> MDEKTKKAEEMALSLARAVAGGDEQAAIKYATWLAEQRVPLRVQVKPEVSPTQDIRLCVSVEDAYMHTVTIWLTVRPDMTVASLKDMVFLDYGFPPSLQQWVVGQRLARDQETLHSHGIRRNGDGAYLYLLSARNTSLNP;> GRQDKMRKEGLQLVSMIQEGETAGASPEEVFSALQYSGTEVPLQWLRSELSYVLEMVAELAGQQDPELGAFSCQEARKAWLDRHGNLDEAVEECVRARRRKVHELQSLGFGPKEGSLQALFQHGGDVARALTELQRQRLEPFHQRLWDRDPEPTPCWD;> GPLGSPEFSSGNFKKEELATRLSQAIAGGDEKAAAQVAAVLAQHHVALNVQLMEAWFPPGPIRLQVTVEDATSVLSSSSSAHVSLKIHPHCSIAALQDQVFSEFGFPPAVQRWVIGRCLCMPERSLASYGVSQDGDPAFLYLLSAPREVSGQSLQNSKMDRKLGLFPQSLGLPHDLQPSSSSLPSPS

The linear ubiquitin chain assembly complex (LUBAC) participates in inflammatory and oncogenic signaling by conjugating linear ubiquitin chains to target proteins. LUBAC consists of the catalytic HOIP subunit and two accessory subunits, HOIL-1L and SHARPIN. In addition, linear ubiquitin chains linked via the N-terminal Met1 are generated by the linear ubiquitin chain assembly complex (LUBAC), which consists of the catalytic HOIP and the accessory HOIL-1L and SHARPIN subunits. Both SHARPIN and HOIL-1L interact with HOIP via their ubiquitin-like (UBL) domains, and the two interactions are thought to sufficiently stabilize LUBAC. We solved the co-crystal structure of the binding regions of the trimeric LUBAC complex and found that LUBAC-tethering motifs (LTMs) located N terminally to the UBL domains of HOIL-1L and SHARPIN heterodimerize and fold into a single globular domain.

Hence, we determined a crystal structure of mHOIP474–630 in ternary complex with mHOIL-1L1–140 and mSHARPIN163–341 at 2.4 Å resolution. As estimated via analytical size-exclusion chromatography, the core subunits assemble into a complex with 1:1:1 stoichiometry. In the ternary complex, mHOIP474–630 adopts an elongated configuration comprising seven a helices and two 310 helices and contains two UBA-like modules, the N-module (aa 474–536; UBA1) and the C-module (aa 559–617; UBA2), tandemly linked through a middle helix α4. The N-terminal μ1 helix in UBA1 and the C-terminal μ7 helix in UBA2 provide the major binding sites for the UBLs of SHARPIN and HOIL-1L, respectively; consequently, in the ternary complex, the two UBLs are independently arranged at opposite ends of the elongated mHOIP D-UBA. Furthermore, the crystal structure of the LUBAC ternary complex core has a new structural motif common to the pre-UBLs of mHOIL-1L and mSHARPIN (residues 5–45 of mHOIL-1L and 170–206 of mSHARPIN), which possess a unique helix-helix-strand structure that mediates stable heterodimerization. Intriguingly, the pair of LTMs folds into a single globular domain, referred to as the ‘‘tethering domain (TD)’’. The major heterodimeric interface in the TD is formed by the hydrophobic faces of the α1 and α2 helices from both LTMs and an intermolecular antiparallel β sheet consisting of the β1 strands (aa 41–45 of mHOIL-1L and 202–206 of mSHARPIN). In the TD, A31 of mHOIL-1L and A192 of mSHARPIN in the α2 helices make a direct van der Waals contact with each other. The TD and HOIP D-UBA undergo no significant interaction, except for a small contact site that could be attributed to crystal packing effects. Taken together, these findings suggest that tethering the UBLs of SHARPIN and HOIL-1L via their LTMs induces a more compact and rigid conformation of HOIP D-UBA than could be achieved by either UBL alone.> KNNINKTRMNDLNREETR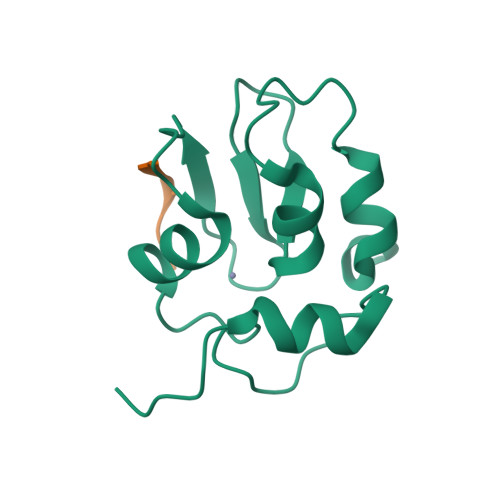LKTFTDWPLDWLDKRQLAQTGMYFTHAGDKVKCFFCGVEIGSWEQEDQPVPEHQRWSPNCPLLRRRTTNNVPINAEALDRILPPISYDICGANDSTLE;> AVAFYIPDQA>MKIADIQVRTEHFPLTRPYRIAFRSIEEIDNLIVEIRTADGLLGLGAASPERHVTGETLEACHAALDHDRLGWLMGRDIRTLPRLCRELAERLPAAPAARAALDMALHDLVAQCLGLPLVEILGRAHDSLPTSVTIGIKPVEETLAEAREHLALGFRVLKVKLCGDEEQDFERLRRLHETLAGRAVVRVDPNQSYDRDGLLRLDRLVQELGIEFIEQPFPAGRTDWLRALPKAIRRRIAADESLLGPADAFALAAPPAACGIFNIKLMKCGGLAPARRIATIAETAGIDLMWGCMDESRISIAAALHAALACPATR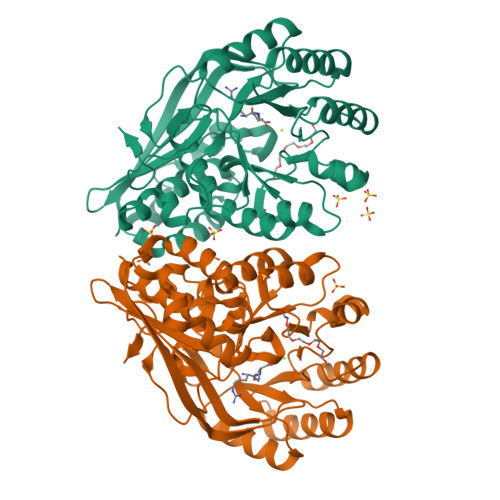YLDLDGSFDLARDVAEGGFILEDGRLRVTERPGLGLVYPD[5x]>[2x]SSPSSPADWAKKLTDAVLRQKAGETLTAADRDFSNADFRNITFSKILPPSFMERDGDIIKGFNFSNSKFTYSDISHLHFDECRFTYSTLSDVVCSNTKFSNSDMNEVFLQYSITTQQQPSFIDTTLKNTLIRHKANLSGVILNEPDNSSPPSVSGGGNFIRLGDIWLQMPLLWTENA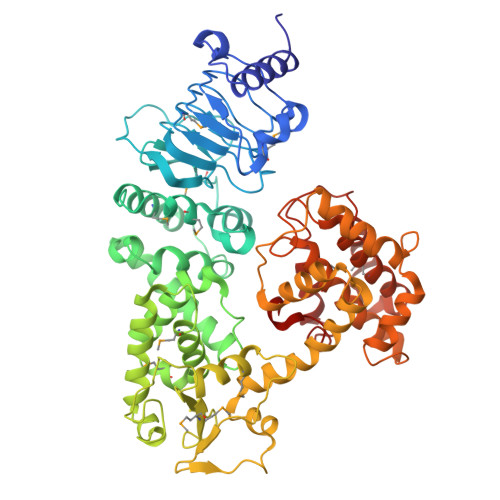VDGFLNHEHNNGKSILMTIDSLPDKYSQEKVQAMEDLVKSLRGGRLTEACIRPVESSLVSVLAHPPYTQSALISEWLGPVQERFFAHQCQTYNDVPLPAPDTYYQQRILPVLLDSFDRNSAAMTTHSGLFNQVILHCMTGVDCTDGTRQKAAALYEQYLAHPAVSPHIHNGLFGNYDGSPDWTTRAADNFLLLSSQDSDTAMMLSTDTLLTMLNPTPDTAWDNFYLLRAGENVSTAQISPVELFRHDFPVFLAAFNQQATQRRFGELIDIILSTEEHGELNQQFLAATNQKHSTVKLIDDASVSRLATIFDPLLPEGKLSPAHYQHILSAYHLTDATPQKQAETLFCLSTAFARYSSSAIFGTEHDSPPALRGYAEALMQKAWELSPAIFPSSEQFTEWSDRFHGLHGAFTCTSVVADSMQRHARKYFPSVLSSILPLAWA> GPVEDVITAAIGRVADTVGTGPTNSEAIPALTAAETGHTSQVVPGDTMQTRHVKNYHSRSESTVENFLCRSACVYFTEYKNSGSKRYAEWVVTTRQAAQLRRKLEFFTYIRFDLELTFVITSTQQPSTTQNQDAQILTHQIMYVPPGGPVPDKVDSYVWQTSTNPSVFWTEGNAPPRMSIPFLSIGNAYSNFYDGWSEFSRNGVYGINTLNNMGTLYARHVNTGSTGPIKSTIRIYFKPKHVKAWIPRPPRLCQYEKAKNVNFQPSGVTTTRQSITTMTNTGAF;> SPTVEECGYSDRVRSITLGNSTITTQECANVVVGYGVWPDYLKDSEATAEDQPTQPDVATCRFYTLDSVQWQKTSPGWWWKLPDALSNLGLFGQNMQYHYLGRTGYTIHVQCNASKFHQGCLLVVCVPEAEMGCATLDNTPSSAELLGGDAAKEFAGEPIASGSNKLVQRVVYNAGMGIGVGNLTIFPHQWINLRTNNSATIVMPYTNSVPMDNMFRHNNITLMVIPFVPLDYCPGSTTYVPITVTIAPMCAEYNGLRLASHQ;> GLPTMNTPGSCQFLTSDDFQSPSAMPQYDVTPEMKIPGEVKNLMEIAEVDSVVPVQNVGEKVNSMEAYQIPVRSNEGSGTQVFGFPLQPGYSSVFSRTLLGEILNYYTHWSGSIKLTFMFCGSAMATGKFLLAYSPPGAGAPTKRVDAMLGTHVVWDVGLQSSCVLCIPWISQTHYRYVASDEYTAGGFITCWYQTNIVVPADAQSSCYIMCFVSACNDFSVRLLKDTPFISQNSFFQ;> MGAQVSTQKTGAHETGLNASGNSIIHYTNINYYKDAASNSATRQDFAQDPGKFTEPVKDIMIKSLPALN;> DCGLPPDVPNAQPALEGRTSFPEDTVITYKCEESFVKIPGEKDSVICLKGSQWSDIEEFCNRSCEVPTRLNSASLKQPYITQNYFPVGTVVEYECRPGYRREPSLS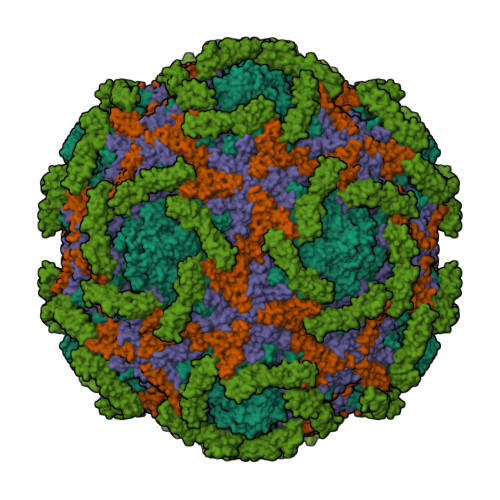PKLTCLQNLKWSTAVEFCKKKSCPNPGEIRNGQIDVPGGILFGATISFSCNTGYKLFGSTSSFCLISGSSVQWSDPLPECREIYCPAPPQIDNGIIQGERDHYGYRQSVTYACNKGFTMIGEHSIYCTVNNDEGEWSGPPPECRGHHHHHH>MGHHHHHHPFRATGDGLFIMNEGNFQYGNATLSYYDPETKKVENEIFYRANAMKLGDVAQSM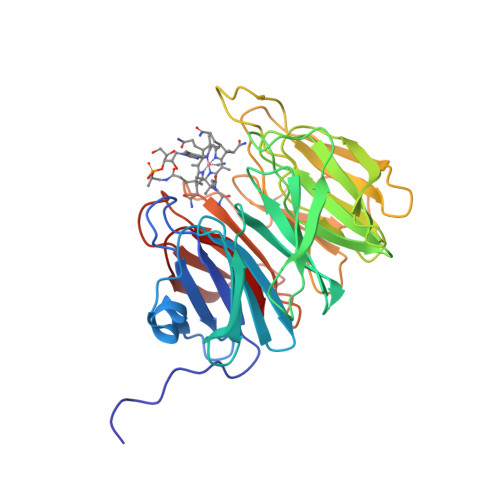IVRDTIGWVVVNNSHVIFAISTNTFKEVGRITGLTSPRYIHFISDEKAYITQIWDYRIFIVNPKTYQITGYIECPDMTMETGSTEQMVQYGKYVYVNCWSYQNRILKIDTTTDKVVDQLTVGIQPTSLVMDKNFKMWTITDGGYKGSPYGYEEPSLYRIDAETFKIEKQFKFQLGDAPSEVQLNGAGDELYWINKDIWRMSVDEERVPVRPFLKYRDTKYYGLTVSPKNGDVYVADAIDYQQQGMIYRYTEDGELVDEFYVGIIPGAFCWK[4x]>GAADHVKGDGKLTSKKISVADYNEIKVDGVIDFNYEQSDDPSTVEVTVDQNLHPYVNIEVKDRVLTIAFKGAKVDHFTKFIVKTNSKWLAAAKVSGNANFMVNSPLTGDETVIKANANSLVQLKETVTVGKLDLNVSGSANMVVNHLEADKIECDIDGSGSITIKKGNAKEGDYSIVSS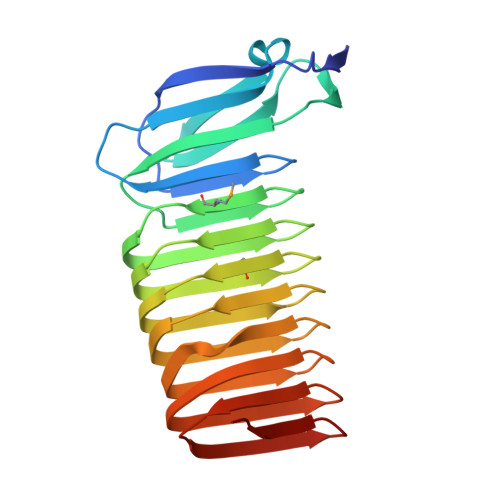GDIHAFGLAVPQLSCKVTGNGLAEVHATDNLKANVVGKGNIRYKGPTAVQQRIIGKGTVEEVKE[3x]>MSEPIHVLITGAAGQIGYALAFRIAKGDLFGDRKVVLHLLEIPPAMKALEGVCMELQDCAFPTLAGVVATDDPEEAFKDVDVAFLVGSFPRKPGMERADLLEKNAGIFKVQGKALSEYAKPTVKVLVVGNPANTNCLIAMANAPKLGPENFSAMTRLDHNRAIGEIAAKLGVPVDKVHNVVVWGNHSNTQVPDVSHATVDKEGGTKKVSDALPKEYLEGEFVQKIAQRGGAVIEARGASSAASAANAALCHMRDWLFGTKPGDWVSMGIPVPEGNPYGIKPGVIYSFPCTVDKDGKVHIVEGLEINDWVREKMEATEKELIEERETAFKVLAQLEHHHHHH[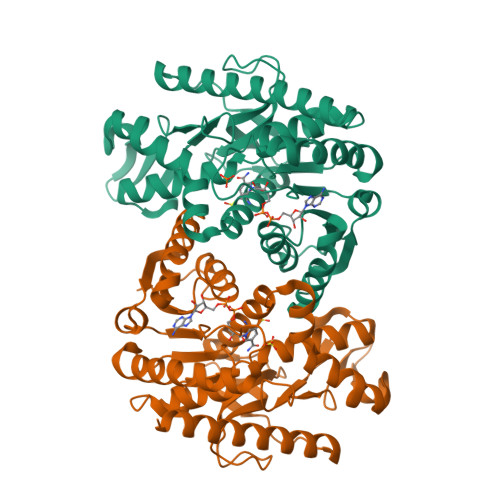2x]>TEKKYIVALDQGTTSSRAVVMDHDANIISVSQREFEQIYPKPGWVEHDPMEIWATQSWTLVEVLAKADISSDQIAAIGITNQRETTIVWEKETGKPIYNAIVWQCRRTAEICEHLKRDGLEDYIRSNTGLVIDPYFSGTKVKWILDHVEGSRERARRGELLFGTVDTWLIWKMTQGRVHVTDYTNASRTMLFNIHTLDWDDKMLEVLDIPREMLPEVRRSSEVYGQTNIGGKGGTRIPISGIAGDQQAALFGQLCVKEGMAKNTYGTGCFMLMNTGEKAVKSENGLLTTIACGPTGEVNYALEGAVFMAGASIQWLRDEMKLINDAYDSEYFATKVQNTNGVYVVPAFTGLGAPYWDPYARGAIFGLTRGVNANHIIRATLESIAYQTRDVLEAMQADSGIRLHALRVDGGAVANNFLMQFQSDILGTRVERPEVREVTALGAAYLAGLAV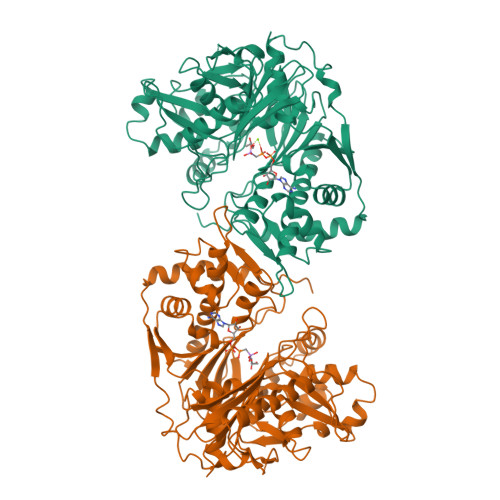GFWQNLDELQEKAVIEREFRPGIETTERNYRYAGWKKAVKRAMAWEEHDE[2x]>GIDPFTAPAVTQHAPYFKGTAVVNGEFKDLSLDDFKGKYLVLFFYPLDFTFVCPTEIVAFSDKANEFHDVNCEVVAVSVDSHFSHLAWINTPRKNGGLGHMNIALLSDLT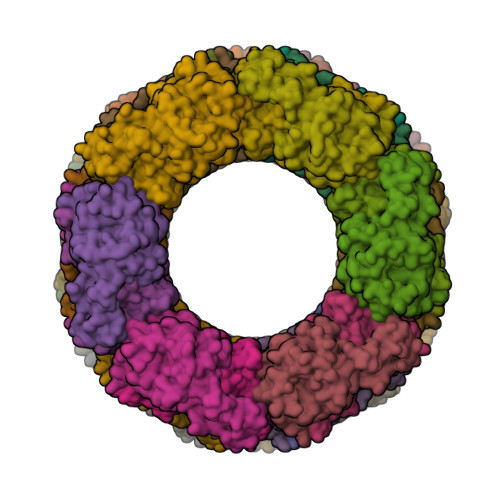KQISRDYGVLLEGSGLALRGLFIIDPNGVIKHLSVNDLPVGRSVEETLRLVKAFQYVETHGEVCPANWTPDSPTIKPSPAASKEYFQKVNQ[9x]>MAGQSTHYLAFPRASTITWGDDTRYWSWATVDFCSYAIEEARLLQVSWLDCRWSMDASDFKQDIWYNASVEVMLTSNASGWNVPLHLEIELPDGSKQESQ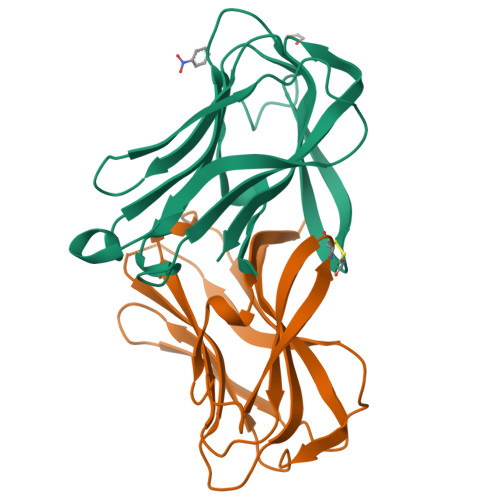IVLAGRQPNVWFKIPIGKFILRGSLTSGTIRFGFYNHEGNWKRGLNIRTLAIQA[2x]> MGNGQGRDWKMAIKRCSNVAVGVGGKSKKFGEGNFRWAIRMANVSTGREPGDIPETLDQLRLVICDLQERREKFGSSKEIDMAIVTLKVFAVAGLLNMTVSTAAAAENMYSQMGLDTRPSMKEAGGKEEGPP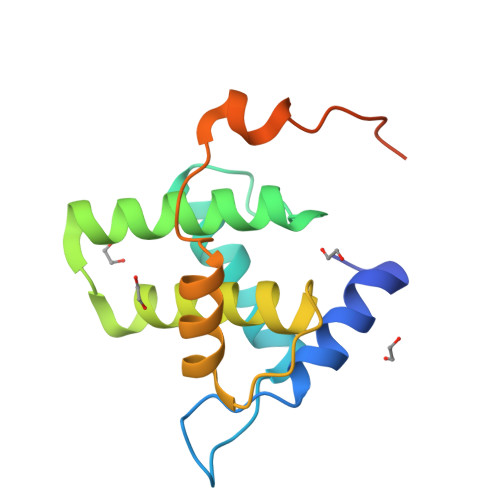QAYLVPRGSLEHHHHHH>GLNYNQEDFMGLDRFFQDAVSHNNTDANAASSIEVEMYECDCMYPT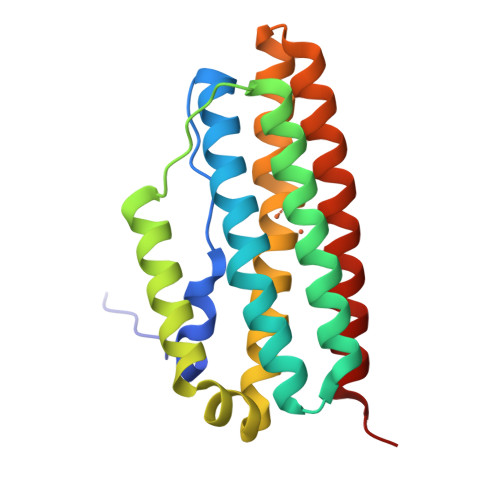FAEIARRSGQPEIGAMFDAIAKEEGMHAQLLTKLYSELEVKDSAETLEAKRLVSTIESQIDAVASDSRGLRRALETALEVETIESQKTYPAFAKLAAEQGNMEVATAFEAIVKSETKHANWVKRALENLLEVA[2x]> GSHMRKIQ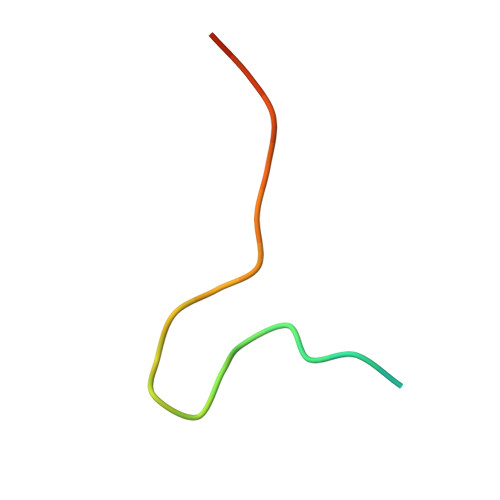RYVRKDGKCNVHHGNVRE>MATLATKKATL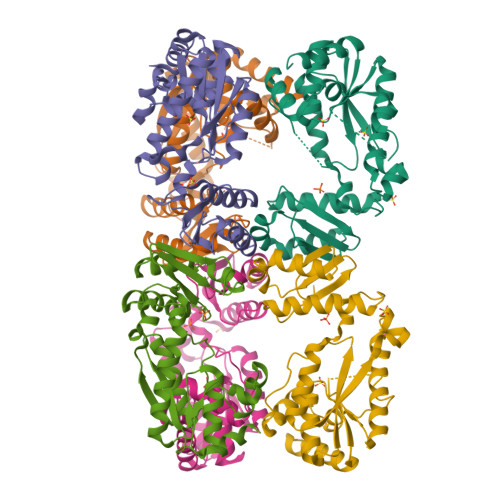VAALKDLQRVTVAFSGGIDSTLVLKMALDVLGRDNVTAVVANSELFTDEEFDKAMSLAEELGANVQGTTLDYLSDDHIKNNTPDSWYYAKKMFYSRLNDIAANNGSAAVLDGMIKNDENDYRPGLKARSEAGARSLLQEADFFKTDVRALAQELGLTNWNKVASCSVSSRFPYGTTLTHDNIAQVMAAEKYLRSLGFPTVRVRFHNDIARIELPEARIGDFLVFNDRVNRQLQSLGFRYVTLDLGGFRSGRMNDTLTKAQLATFAASWSHPQFEK[6x]>GSHMASLNLENKTYVIMGIANKRSIAFGVAKVLDQLGAKLVFTYRKERSRKELEKLLEQLNQPEAHLYQIDVQSDEEVINGFEQIGKDVGNIDGVYHSIAF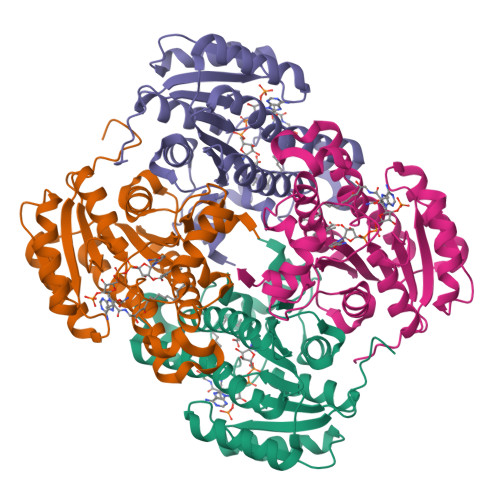ANMEDLRGRFSETSREGFLLAQDISSYSLTIVAHEAKKLMPEGGSIVATTYLGGEFAVQNYNVMGVAKASLEANVKYLALDLGPDNIRVNAISAGPIRTLSAKGVGGFNTILKEIEERAPLKRNVDQVEVGKTAAYLLSDLSSGVTGENIHVDSGFHAIK[8x]> GPLGSMPSQMEHAMETMMFTFHKFAGDKGYLTKEDLRVLMEKEFPGFLENQKDPLAVDK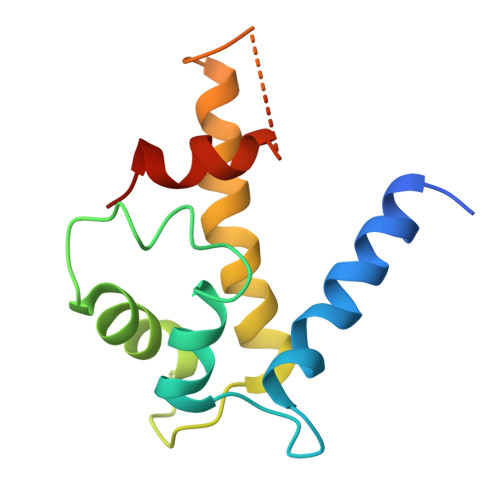IMKDLDQCRDGKVGFQSFFSLIAGLTIACNDYFVVHMKQENLYFQGDSTVHEILSKLSLEGD> MSLKKALFLILDQYADWEGVYLASALNQREDWSVHTVSLDPIVSSIGGFKTSVDYIIGLEPANFNLLVMIGGDSWSNDNKKLLHFVKTAFQKNIPIAAICGAVDFLAKNGLLNNHSHTGNFVYLWKDYKQYKPISSFVEKQAVRDKNLVTANGTAP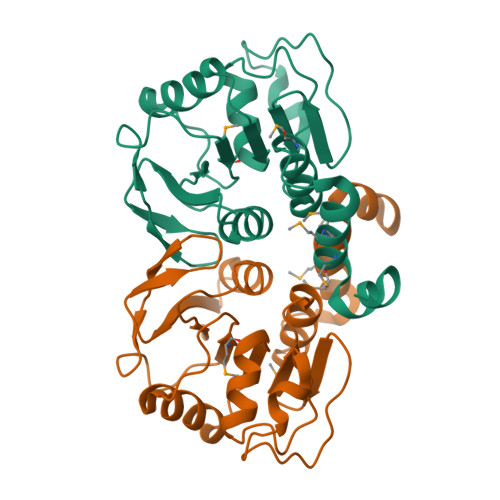IEFTNLILEMIDFDTPENIEKMMYMNRYGFYHFCDKYGNPFVEGHHHHHH>[2x]A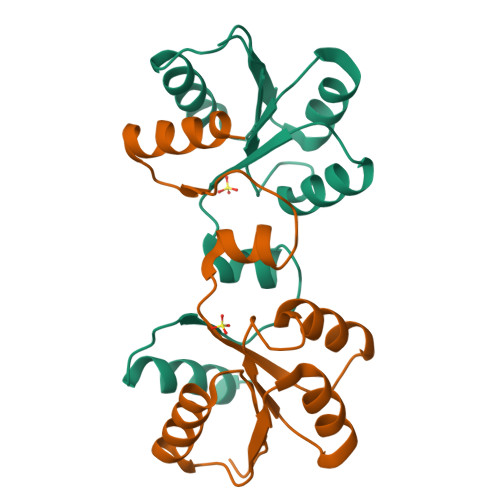ATNILIVEDDPMVQFIHRNYLEKIGTFDTIYSSETIADAKKLLASRSIQLVLLAIRLKDGNGIDFLTDLRRTKQTVDVILITAANEVNIVNDALHLGVIDYLIKPFTLERFEKSIQRYRTK>MSQSQRSTADWQRLDAAHHLHPFTDYGELNTKGSRIITRAEGCYLWDSDGNQILDGMAGLWCVNIGYGRKELAEVAYRQMQELPYYNNFFQCSHPPAIELSRLLSEVTPKHMNHVFFTGSGSDSNDTILRMVRYYWKLLGKPYKKVVISRENAYHGSTVAGASLSGMKAMHSHGDLPIPGIEHIEQPYHFGRAPDMDPAEFGRQAAQALERKIDEIGECNVAAFIAEPIQGAGGVIIPPDSYWPEIKRICAERDILLIVDEVITGFGRLGTWFGSQYYDLQPDLMPIAKGLSSGYMPIGGVMVSDRVAKVVIEEGGEFFHGYTYSGHPVAAAVAAENIRIMRDEGIIERAGA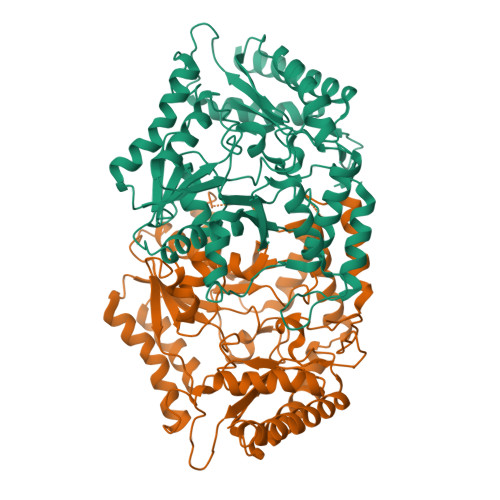EIAPYLQARWRELGEHPLVGEARGVGMVAALELVKSKQPLERFEEPGKVGSLCRDLSVKNGLVMRAVGGTMIISPPLVLSREQVDELIDKARRTLDETHKAIGGALEHHHHHH[4x]>GAMGSMKIGIIAAMEEELSLLLANLLDAQEHQVLSKTYYTGRFGKHELILVQSGVGKVMSAMTVAILVEHFKAQAIINTGSAGAVASHLAIGDVVVADRLVYHDVDATAFGYAYGQMAGQPLYYDCDPQFVAIFKQVLKHEKTNGQVGLIATGDSFVAGQDKIDQIKTAFSNVLAVEMEGAAIAQAAHTAGKPFIVVRAMSDTAAHDANITFDQFIIEAGKRS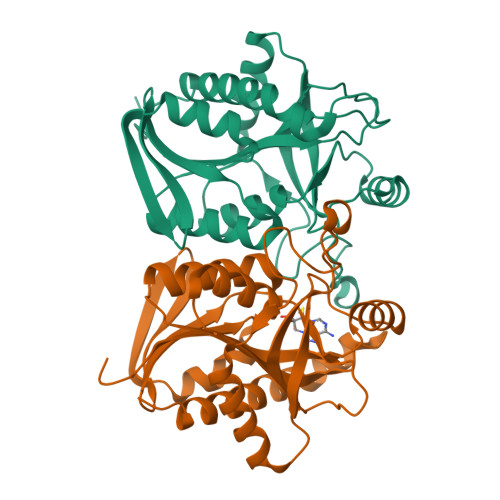AQILMTFLENLPV[2x]1-(1-BENZOTHIOPHEN-3-YL)METHANAMINE | C9 H9 N S | 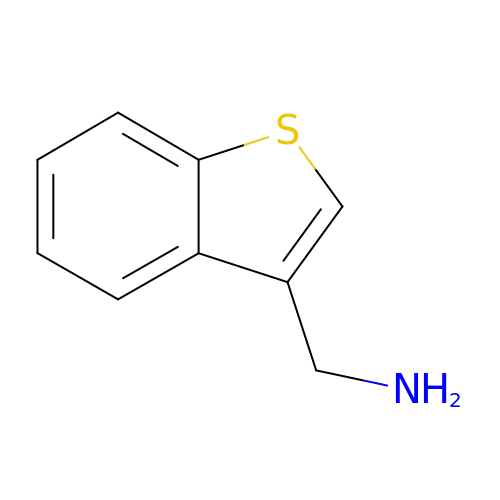WHTPXNOFEHTZAD-UHFFFAOYSA-N>[14x]MISPEQAMRERSELARKGIARAKSVVALAYAGGVLFVAENPSRSLQKISELYDRVGFAAAGKFNEFDNLRRGGIQFADTRGYAYDRRDVTGRQLANVYAQTLGTIFTE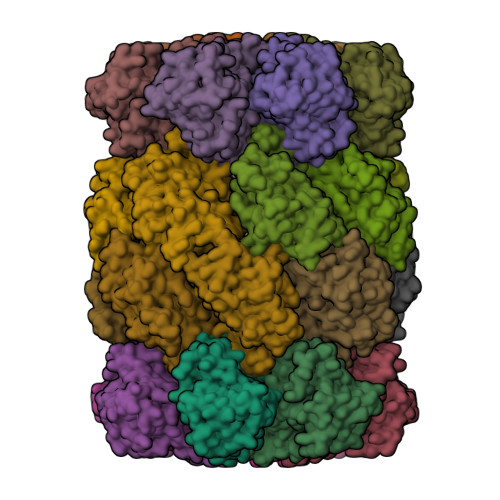QAKPYEVELCVAEVAHYGETKRPELYRITYDGSIADEPHFVVMGGTTEPIANALKESYAENASLTDALRIAVAALRAGSADTSGGDQPTLGVASLEVAVLDANRPRRAFRRITGSALQALLVDQESPQSDGESSG;>TTIVALKYPGGVVMAGDRRSTQGNMISGRDVRKVYITDDYTATGIAGTAAVAVEFARLYAVELEHYEKLEGVPLTFAGKINRLAIMVRGNLAAAMQGLLALPLLAGYDIHASDPQSAGRIVSFDAAGGWNIEEEGYQAVGSGSLFAKSSMKKLYSQVTDGDSGLRVAVEALYDAADDDSATGGPDLVRGIFPTAVIIDADGAVDVPESRIAELARAIIESRSGADTFGSDGGEK[14x]>GHMNKDNLRSPICCILGHVDTGKTKLLDKIRQTNVQEGEAGGITQQIGATYFPVEAIKQKTAVVNKDGKFEFKVPGLLIIDTPGHESFSNLRSRGSSLCNIAILVVDIMHGLEPQTIESLRLLRERKTPFVVALNKIDRLYGWKKIENNGFRESFALQNKAVQNEFRNRLDQVKLQFAEQGFNSELFYENKNFARYVSLVPTSAHTGEGIPDMLKLIVQLCQERMASSLMYLSELQATVLEVKAIEGFGVTIDVILSNGILREGDRIVLCGLEGPIKTNIRALLTPAPMRELRIKGQYIHHKEVKAAQGVKISA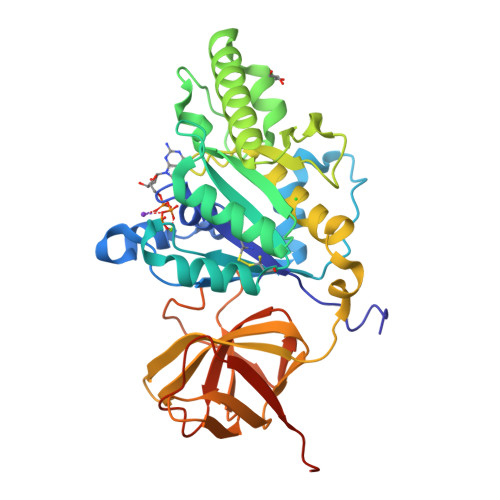PGLEGAIAGSRLLVVGPDDDEEELEEEVESD[2x]>[10x]APADNAADARPVD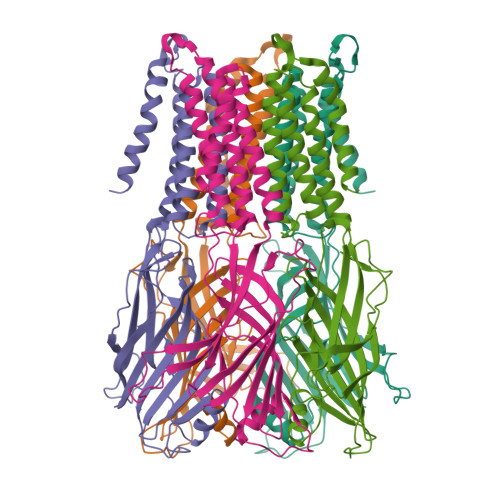VSVSIFINKIYGVNTLEQTYKVDGYIVAQWTGKPRKTPGDKPLIVENTQIERWINNGLWVPALEFINVVGSPDTGNKRLMLFPDGRVIYNARFLGSFSNDMDARLFPFDRQQFVLELEPFSYNNQQLRFSDIQVYTENIDNEEIDEWWIRGKASTHISDIRYDHLSSVQPNQNEFSRITVRIDAVRNPSYYLWSFILPLGLIIAASWSVFWLESFSERLQTSFTLMLTVVAYAFYTSNILPRLPYTTVIDQMIIAGYGSIFAAILLIIFAHHRQANGVEDDLLIQRCRLAFPLGFLAIGCVLVIRGITL> MAGWQSYVDNLMCDGCCQEAAIVGYCDAK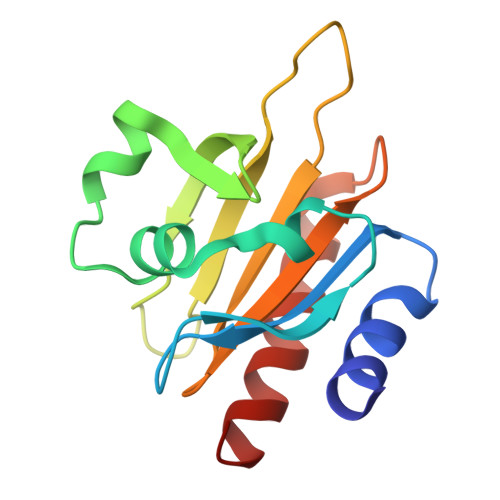YVWAATAGGVFQSITPVEIDMIVGKDREGFFTNGLTLGAKKCSVIRDSLYVDGDCTMDIRTKSQGGEPTYNVAVGRAGRVLVFVMGKEGVHGGGLNKKAYSMAKYLRDSGF TETRADECANOYL-COA | C35 H62 N7 O17 P3 S | 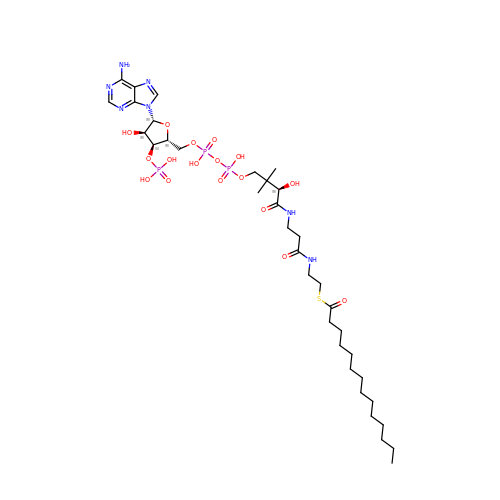DUAFKXOFBZQTQE-QSGBVPJFSA-N>[4x]GMSEPYTWKSVVTGAGGGF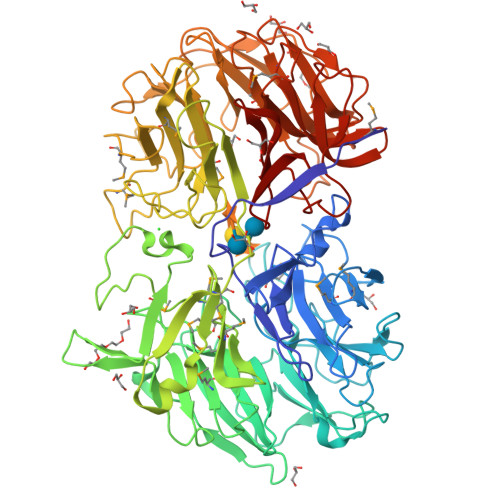VPGIIFNQTEPNLIYARTDIGGAYRWNQATSSWVSISDSVGWVDWNKNGVDALATDPIDPNKVYMATGTYTNHWDNNGQIMRSNDRGNTWQTTPLPFKVGGNMPGRSAGERLVIDPNKNNILYFGARSGNGLWKSIDSGVTWSKVTSFPNVGTYIQNPTLDYGNDLVGLSWITFDKSTGTLGNATQTIYVGVADTASSVYRSTDGGVTWTALAGQPTGFLPHHGELSSTGDLYITYSNGVGPYDGSKGEVWKYNKTSGAWTNISPTTGTDNWYGFGGLALDAQHPNTLMVSSLNAWWPDEVIFRSTNGGATWSRIWDWGNYPERTYKFSMDITAAPWLDHGTTSTSLDPSPKLGWMMGDLEIDPFNSNRMMYGTGATIYGSNNLTSWDTGGKVNISVMAKGVEETAVLGLISPPTGTSHLITALGDVSGFRHEDLSVAPTKFQTSPSWATTMSIDYAELSPSYMVRVGSADKEKTPSMKSIGISNDGGVNWYMPNSEPSNGTKTTVGHGQVAVSASGNSILWSTSDIGVYYSKTSGNSWTASAGLPAGAKIASDRVNPNKYYGFYAGTFYVSVDGGATFTATGASGFPTNNVAGLQPNEAQISMKAVPGIEGDIWFAGGNTVENKYGLWHSTNSGASFTKLTNVEEADLIGYGKAAPGQTYMSLYTVAKIDGVRGVFRSDDVGATWVRINDDAHQYAKINMAITGDPRIYGRVYLGTNGRGTLYADPV>SVLQVLHIPDERLRKVAKPVEEVNAEIQRIVDDMFETMYAEEGIGLAATQVDIHQRIIVIDVSENRDERLVLINPELLEKSGETGIEEGCLSIPEQRALVPRAEKVKIRALDRDGKPFELEADGLLAICIQHEMDHLVGKLFMDYLSPLKQQRIRQKVEKLDRL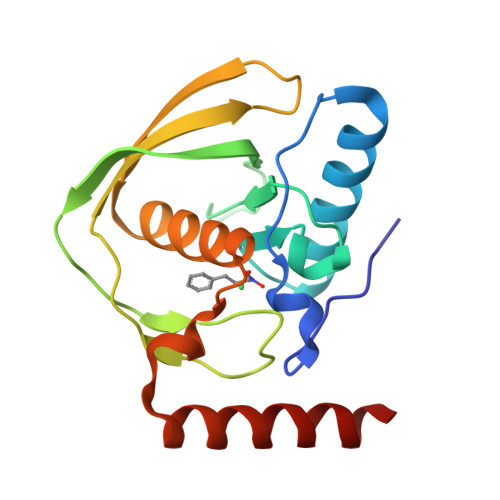KARA[3x]> MGAQLSLVVQASPSIAIFSYIDVLEEVHYVSQLNSSRFLKTCKALDPNGEIVIKVFIKPKDQYSLRPFLQRIRAQSFKLGQLPHVLNYSKLIETNRAGYMIRQHLKNNLYDRLSLRPYLQDIELKFIAFQLLNALKDIHNLNIVHGDIKTENILVTSWNWCILTDFAAFIKPVYLPEDNPGEFLFYFDTSKRRTCYLAPERFNSKLYQDGKSNNGRLTKEMDIFSLGCVIAEIFAEGRPIFNLSQLFKYKSNSYDVNREFLMEEMNSTDLRNLVLDMIQLDPSKRLSCDELLNKYRGIFFPDYFYTFIYDYFRNLVTMTTSTPISDNTCTNSTLEDNVKLLDETTEKIYRDFSQICHCLDFPLIKDGGEIGSDPPILESYKIEIEISRFLNTNLYFP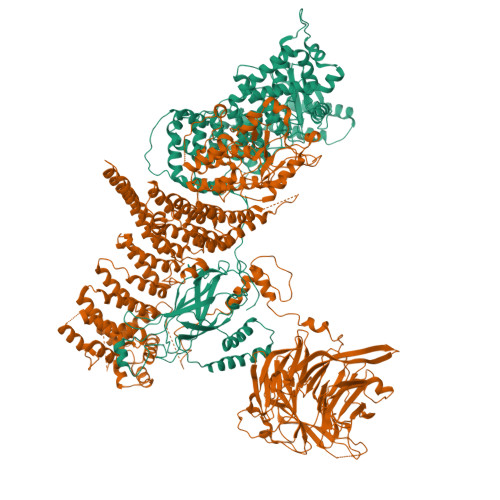QNYHLVLQQFTKVSEKIKSVKEECALLFISYLSHSIRSIVSTATKLKNLELLAVFAQFVSDENKIDRVVPYFVCCFEDSDQDVQALSLLTLIQVLTSVRKLNQLNENIFVDYLLPRLKRLLISNRQNTNYLRIVFANCLSDLAIIINRFQEFTFAQHCNDNSMDNNTEIMESSTKYSAKLIQSVEDLTVSFLTDNDTYVKMALLQNILPLCKFFGRERTNDIILSHLITYLNDKDPALRVSLIQTISGISILLGTVTLEQYILPLLIQTITDSEELVVISVLQSLKSLFKTGLIRKKYYIDISKTTSPLLLHPNNWIRQFTLMIIIEIINKLSKAEVYCILYPIIRPFFEFDVEFNFKSMISCCKQPVSRSVYNLLCSWSVRASKSLFWKKIITNHVDSFGNNRIEFITKNYSSKNYGFNKRDTKSSSSLKGIKTSSTVYSHDNKEIPLTAEDRNWIDKFHIIGLTEKDIWKIVALRGYVIRTARVMAANPDFPYNNSNYRPLVQNSPPNLNLTNIMPRNIFFDVEFAEESTSEGQDSNLENQQIYKYDESEKDSNKLNINGSKQLSTVMDINGSLIFKNKSIATTTSNLKNVFVQLEPTSYHMHSPNHGLKDNANVKPERKVVVSNSYEGDVESIEKFLSTFKILPPLRDYKEFGPIQEIVRSPNMGNLRGKLIATLMENEPNSITSSAVSPGETPYLITGSDQGVIKIWNLKEIIVGEVYSSSLTYDCSSTVTQITMIPNFDAFAVSSKDGQIIVLKVNHYQQESEVKFLNCECIRKINLKNFGKNEYAVRMRAFVNEEKSLLVALTNLSRVIIFDIRTLERLQIIENSPRHGAVSSICIDEECCVLILGTTRGIIDIWDIRFNVLIRSWSFGDHAPITHVEVCQFYGKNSVIVVGGSSKTFLTIWNFVKGHCQYAFINSDEQPSMEHFLPIEKGLEELNFCGIRSLNALSTISVSNDKILLTDEATSSIVMFSLNELSSSKAVISPSRFSDVFIPTQVTANLTMLLRKMKRTSTHSVDDSLYHHDIINSISTCEVDETPLLVACDNSGLIGIFQ;> MSLNNITFCVSQDLDVPLKVKIKSLEGHKPLLKPSQKILNPELMLIGSNVFPSSDLIVSLQVFDKERNRNLTLPIYTPYIPFRNSRTWDYWLTLPIRIKQLTFSSHLRIILWEYNGSKQIPFFNLETSIFNLKDCTLKRGFESLKFRYDVIDHCEVVTDNKDQENLNKYFQGEFTRLPWLDEITISKLRKQRENRTWPQGTFVLNLEFPMLELPVVFIEREIMNTQMNIPTLKNNPGLSTDLREPNRNDPQIKISLGDKYHSTLKFYDPDQPNNDPIEEKYRRLERASKNANLDKQVKPDIKKRDYLNKIINYPPGTKLTAHEKGSIWKYRYYLMNNKKALTKLLQSTNLREESERVEVLELMDSWAEIDIDDALELLGSTFKNLSVRSYAVNRLKKASDKELELYLLQLVEAVCFENLSTFSDKSNSEFTIVDAVSSQKLSGDSMLLSTSHANQKLLKSISSESETSGTESLPIVISPLAEFLIRRALVNPRLGSFFYWYLKSESEDKPYLDQILSSFWSRLDKKSRNILNDQVRLINVLRECCETIKRLKDTTAKKMELLVHLLETKVRPLVKVRPIALPLDPDVLICDVCPETSKVFKSSLSPLKITFKTTLNQPYHLMFKVGDDLRQDQLVVQIISLMNELLKNENVDLKLTPYKILATGPQEGAIEFIPNDTLASILSKYHGILGYLKLHYPDENATLGVQGWVLDNFVKSCAGYCVITYILGVGDRHLDNLLVTPDGHFFHADFGYILGQDPKPFPPLMKLPPQIIEAFGGAESSNYDKFRSYCFVAYSILRRNAGLILNLFELMKTSNIPDIRIDPNGAILRVRERFNLNMSEEDATVHFQNLINDSVNALLPIVIDHLHNLAQYWRT> MAGRAQIPTKS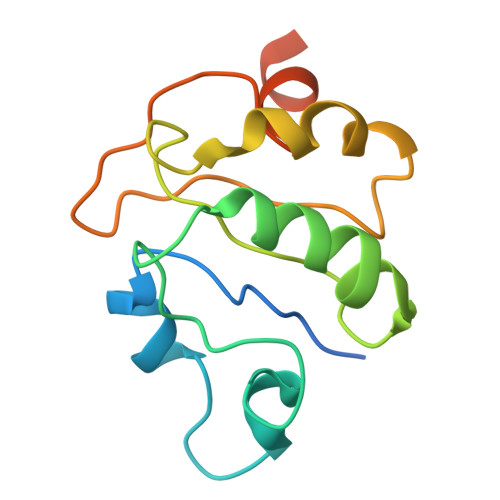SALIAMIADEDTVTGFLLAGVGNVDLRRKTNYLIVDSKTTVKAIEDAFKEFTTKEDIAIVLISQYVANMIRFLVDSYNKPIPAILEIPSKDHPYDPAHDSVLSRVKNLFSAESVASGRR>[2x]GAMEEETFYSVRMRASMNGSHEDGGKHISGGERLIPFHEMKHTVNALLEKGLSHSRGKPDFMQIQFEEVHESIKTIQPLPVHTNEVSCPEEGQKLARLLLEKEGVSRDVIEKAYEQIPEWSDVRGAVLFDIHTGKRMDQT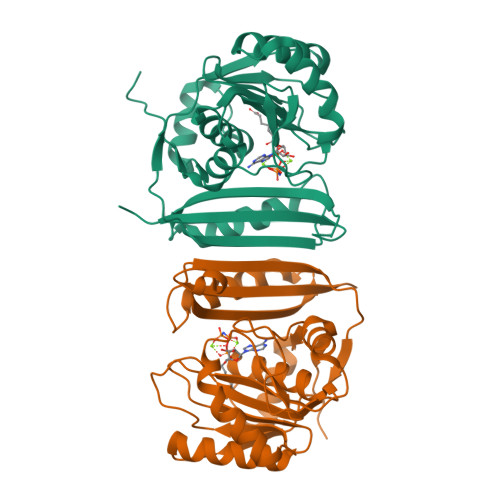KEKGVRVSRMDWPDANFEKWALHSHVPAHSRIKEALALASKVSRHPAVVAELCWSDDPDYITGYVAGKKMGYQRITAMKEYGTEEGCRVFFIDGSNDVNTYIHDLEKQPILIEWEEDHDS>MGSSHHHHHHGSLSKQIPLGIYEKALPAGECWLERLQLAKTLGFDFVEMSVDETDERLSRLDWSREQRLALVNAIVETGVRVPSMCLSAHRRFPLGSEDDAVRAQGLEIMRKAIQFAQDVGIRVIQLAGYDVYYQEANNETRRRFRDGLKESVEMASRAQVTLAMEIMDYPLMNSISKALGYAHYLNNPWFQLYPDIGNLSAWDNDVQMELQAGIGHIVAVHVKDTKPGVFKNVPFGEGVVDFERCFETLKQSGYCGPYLIEMWSETAEDPAAEVAKARDWVKARMAKAGMVEA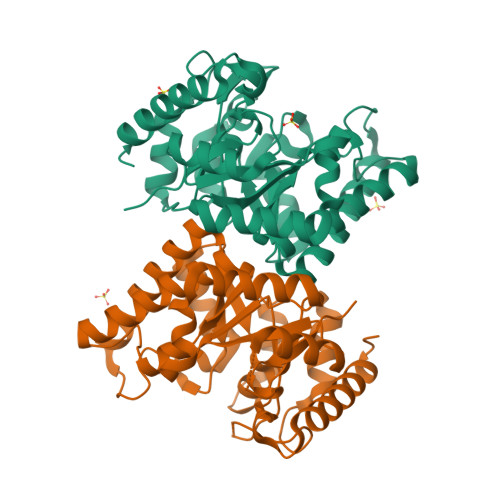A[2x]> MTRFAEKVAIITGSSNGIGRATAVLFAREGAKVTITGRHAERLEETRQQILAAGVSEQNVNSVVADVTTDAGQDEILSTTLGKFGKLDILVNNAGAAIPDSQSKTGTAQSIESYDATLNLNLRSVIALTKKAVPHLSSTKGEIVNISSIASGLHATPDFPYYSIAKAAIDQYTRNTAIDLIQHGIRVNSISPGLVATGFGSAMGMPEETSKKFYSTMATMKECVPAGVMGQPQDIAEVIAFLADRKTSSYIIGHQLVVDGGSSL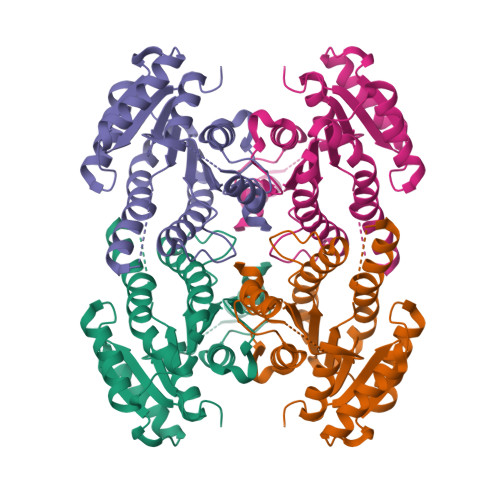IMGLHCQDFAKLLH>[2x]EVNLDRYQTALEEVLSWLLSAEDTLQAQGEISNDVEVVKDQFHTHEGYMMDLTAHQGRVGNILQLGSKLIGTGKLSEDEETEVQEQMNLLNSRWECLRVASMEKQSNLHRVLMDLQNQK

Dystrophin is a large (427 kD) multidomain protein expressed in skeletal and cardiac muscle where it binds to the dystrophin-associated glycoprotein (DAG) complex of the plasma membrane and to F-actin connecting the cytoskeleton to the membrane. Utrophin (Utr), the 395 kD autosomal homologue of Dys is widely expressed in non muscle tissues (reviewed) but is restricted to the myotendinous and neuromuscular junctions of differentiated muscle and is located at the sarcolemma of developing fetal muscle. Dys and Utr potentially act as cellular biomechanical shock-absorbers limiting damage to the plasma membrane with the spectrin repeat domains acting as spring units by undergoing force-induced unfolding. Dys and Utr-SR1 adopt the canonical spectrin repeat fold comprising a triple helical bundle displaying an approximately cylindrical structure of overall dimensions ∼60 Å length and ∼9 Å radius (between backbone atoms).

The Dys N-terminal (repeat 1) spectrin repeat (Dys-SR1) also crystallized with two molecules in the asymmetric unit but there is no relationship between the two crystal symmetries. Based on sequence analysis Dys repeat 1 has been previously defined as amino acids 338–446/7. Comparing the structure of Dys-SR1 with Utr-SR1 results in rmsds of 0.8–1.9 Å (112 Cα) depending on which of the four molecules in the asymmetric unit of the two crystals are superimposed in a pair-wise manner. Dys-SR1A and Utr-SR1 (A & B) form the more typical conserved interaction between W354/W324 with helix B H392/H362 and helix C W431/W401. Instead of forming the usually conserved interactions with H392 (heptad ‘d’ position, helix B) and W431 (‘a’, helix C) Dys-SR1B W354 stacks against R395, one helical turn distant from 392, and is associated with both a twisting of the bend region in the centre of helix B and a crystal contact (M387 distance 3.5 Å) from a crystallographically-related molecule. This disruption of sidechain interactions relaxes the Dys-SR1B main chain so that canonical helical main chain hydrogen bonds are formed in contrast to Dys-SR1 monomer A and Utr-SR1.>MATGHTDPQRRERILAATLDLIAEEGIARVSHRRIAQRAGVPLGSMTYHFTGIEQLLREAFGRFTDHIVAVFDEHLGAAADRDEAREAVADLVHELSEDSQRDLVLTQELYTLAARQPAYRELTHEWMRRSRVHLEKHF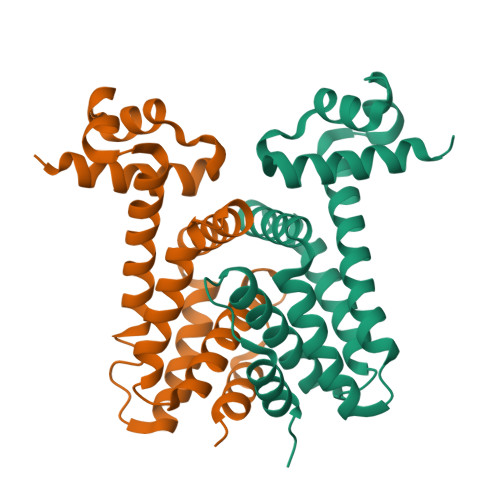DPGTARQLDALIEGLTLHRALAREPHGRALTLEAIARITTTDRPAPLEHHHHHH[4x]(~{Z})-2-oxidanylbut-2-enedioic acid | C4 H4 O5 | 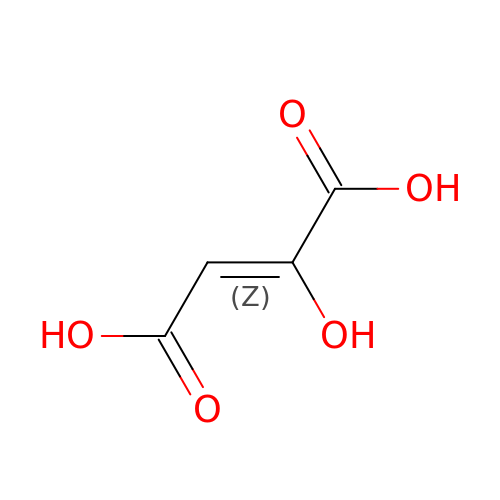UWYVPFMHMJIBHE-UPHRSURJSA-N> GPGSMERRLGVRAWVKENRGSFQPPVCNKLMHQEQLKVMFIGGPNTRKDYHIEEGEEVFYQLEGDMVLRVLEQGKHRDVVIRQGEIFLLPARVPHSPQRFANTVGLVVERRRLETELDGLRYYVGDTMDVLFEKWFYCKDLGTQLAPIIQEFFSSEQYRTGKPIPDQLL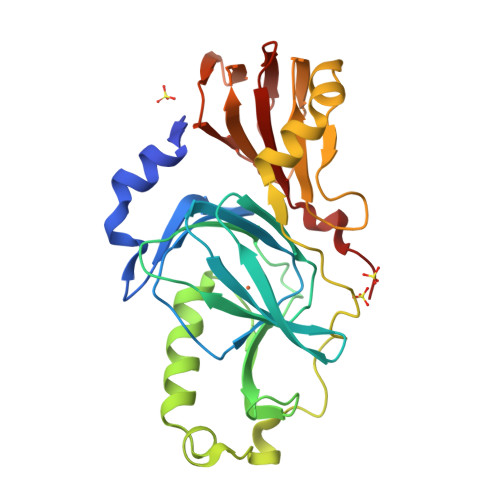KEPPFPLSTRSIMEPMSLDAWLDSHHRELQAGTPLSLFGDTYETQVIAYGQGSSEGLRQNVDVWLWQLEGSSVVTMGGRRLSLAPDDSLLVLAGTSYAWERTQGSVALSVTQDPACKKPLG>MKLSKDTIAILKNFASINSGILLSQGKFIMTRAVNGTTYAEANISDEIDFDVALYDLNSFLSILSLVSDDAEISMHTDGNIKIADTRSTVYWPAADKSTIVFPNKPIQFPVASVITEIKAEDLQQLLRVSRGLQIDTIA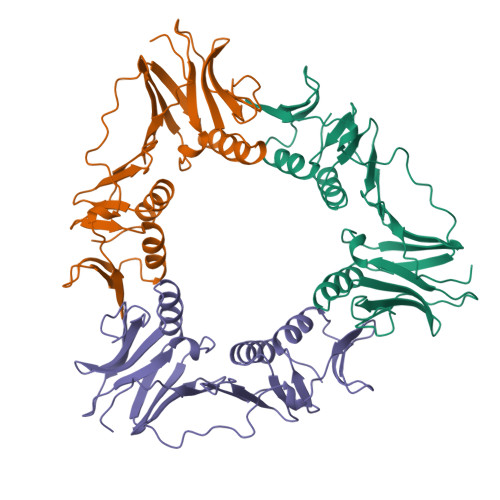ITNKDGKIVINGYNKVEDSGLTRPKYSLTLTDYDGSNNFNFVINMANMKIQPGNYKVMLWGAGDKVAAKFESSQVSYVIAMEADSTHDF[3x]>NEKGERISMINPRVVLDENGISHRSRYFIMLCDNETAIAHAKKTSIWAVKKDSSKRISDAYKKASVYFIFVAQQTYNALGYAQVVSDLNSTELPFWSDSSHAGGVRIKWIKTCNLFSAEISEIVS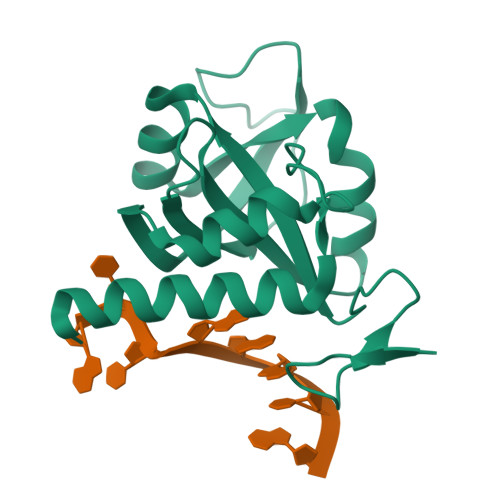HMDHGSEARDGMEMMYDEGSRLCTLINYAIMKRIGRDR[2x]> XATSRYEPVAEIGVGAYGTVYKARDPHSGHFVALKSVRVPNGGGGGGGLPISTVREVALLRRLEAFEHPNVVRLMDVCATSRTDREIKVTLVFEHVDQDLRTYLDKAPPPGLPAETIKDLMRQFLRGLDFLHANCIVHRDLKPENILVTSGGTVKLADFGLARIYSYQMALTPVVVTLWYRAPEVLLQSTYATPVDMWSVGCIFAEMFRRKPLFCGNSEADQLGKIFDLIGLPPEDDWPRDVSLPRGAFPPRGPRPVQSV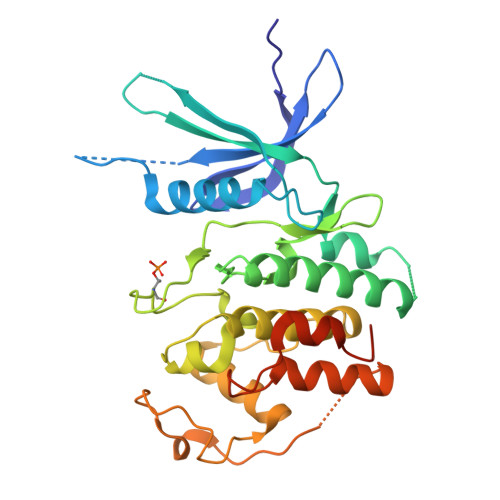VPEMEESGAQLLLEMLTFNPHKRISAFRALQHSYLHKDEGNPEEGHHHHHH> MALRGVPIRLGVHRVGYTHPSTLPVPCAQRWDLRLARARIFQEYIEEKAPGAWQLEDERSMSPEFKTFTGYPMREMRPGYGQNLPDFIMKKRLPNNTHYELFARRDIPNEDNAMYGKYLYDMTVHGT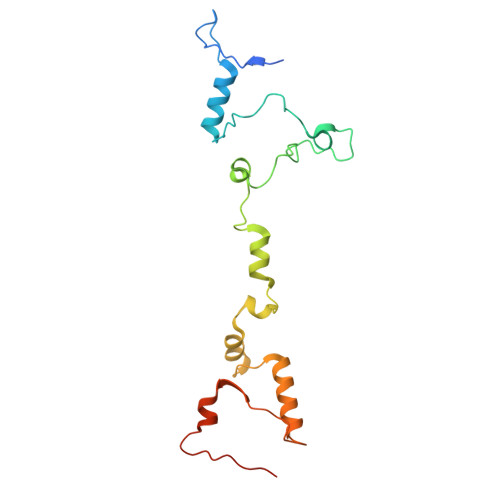SLPSTYRMHKDINKAQRNDRKLSGNRFRVLCSSGAKKPPSGWEPIPDATEEEE> SNAPFKESQARGLLQDNMANSYNGGDFEDGLLNLSKEVFPTDKYLYQDGQFLDKKTINAYLNPKYTKREIDKMSEKDKKDKKANENLGLNPSHEGETNPEKIAEKSPAYLSNILEQDFYGGGDT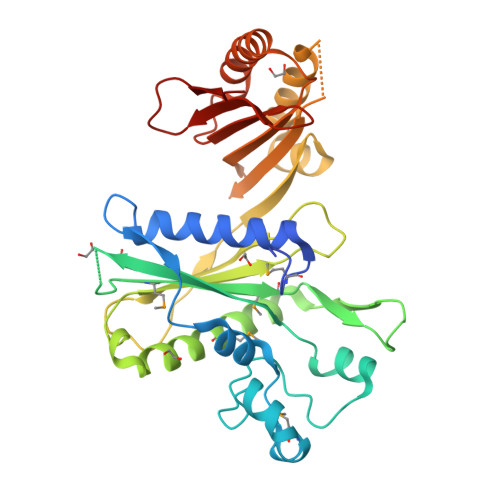KGKNIKGMTIGLAMNSVYYYKKEKDGPTFSKKLDDSEVKKQGKQMASEILSRLRENDDLKDIPIHFAIYKQSSEDSITPGEFITQATAEKSQTKLNEWHNINEKSALLPSSTAADYDENLNNNFKQFNDNLQSYFSNFTQAVGKVKFVDKKPQRLVVDLPIDYYGQAETIGITQYVTEQANKYFDKIDNYEIRIKDGNQPRALISKTKDDKEPQVHIYSN>[8x]MSQQPGVLPENMKRYMGRDAQRMNILAGRIIAETVRSTLGPKGMDKMLVDDLGDVVVTNDGVTILREMSVEHPAAKMLIEVAKTQEKEVGDGTTTAVVVAGELLRKAEELLDQNVHPTIVVKGYQAAAQKAQELLKTIACEVGAQDKEILTKIAMTSITGKGAEKAKEKLAEIIVEAVSAVVDDEGKVDKDLIKIEKKSGASIDDTELIKGVLVDKERVSAQMPKKVTDAKIALLNCAIEIKETETDAEIRITDPAKLMEFIEQEEKMLKDMVAEIKASGANVLFCQKGIDDLAQHYLAKEGIVAARRVKKSDMEKLAKATGANVITNIKDLSAQDLGDAGLVEERKISGDSMIFVEECKHPKAVTMLIRGTTEHVIEEVARAVDAAVGVVGCTIEDGRIVSGGGSTEVE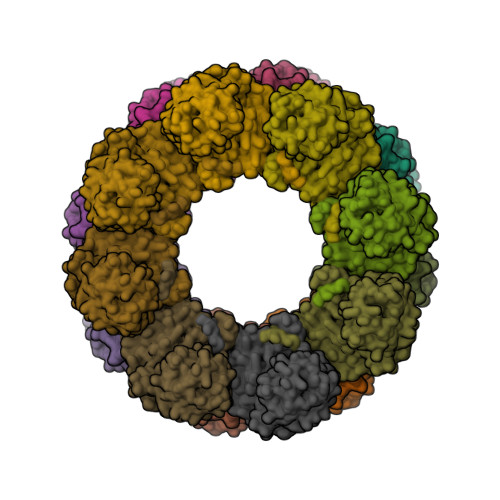LSMKLREYAEGISGREQLAVRAFADALEVIPRTLAENAGLDAIEILVKVRAAHASNGNKCAGLNVFTGAVEDMCENGVVEPLRVKTQAIQSAAESTEMLLRIDDVIAAEKLRGAPDMGDMGGMPGMGGMPGMM(3S,5Z,7E,22E)-9,10-secoergosta-5,7,10,22-tetraen-3-ol 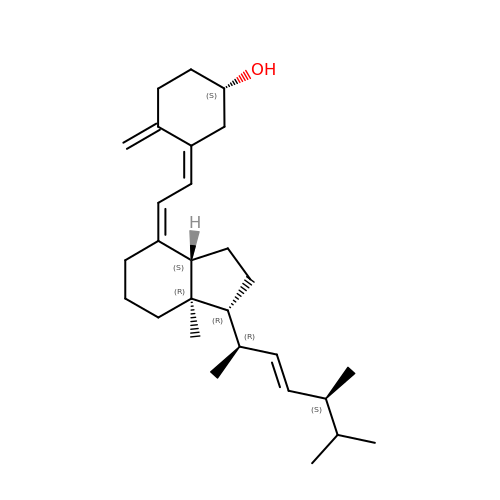| C28 H44 O | MECHNRXZTMCUDQ-RKHKHRCZSA-N>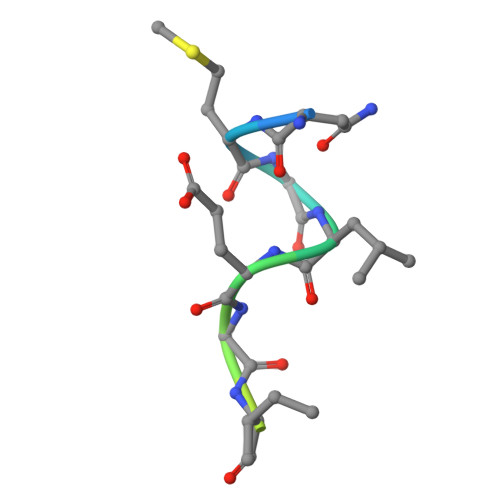 TNMGLEAIIRKALMGK>[2x]MGSSHHHHHHLEVLFQGPAGSMATERDQEIIDFIDQGNYTYAQSLITKKLAKSPQKLFYHVLQNEIHLKSGQRELAIKKNLELLNRYPNDPLTIEKLSDFFSKMEMEKESSLVYENAIKKYPVSTETLCLSWFDNSIEKYDFKVFNRIFMYLNKNGKSRLHTLWYAFSFHLLLQEGETDKASLYNSLGKKLMEGLQPFENTQEIYVYTLFLSSKEIEQVLSGVTLPLDLELKLLYMKAMKENASFEALHAYTEKLLFKEKFDDFDTWKLWILSGKEIGKSFEELDQKLTLPTRNISLLKIELDILYSRNIETSVENYYQKFNTKLCCYADLSQYELPTSFIGSLKNSTSEENLITVVNNRKFVNQTDNWDVYERFSTKEGAEYDSNPVNELTLRTIVSDLDSSPQNTIKNIVLLKHLLEQDKYNYKLKLWLMKLYSQLNTNDLIFPIYNGLKIRM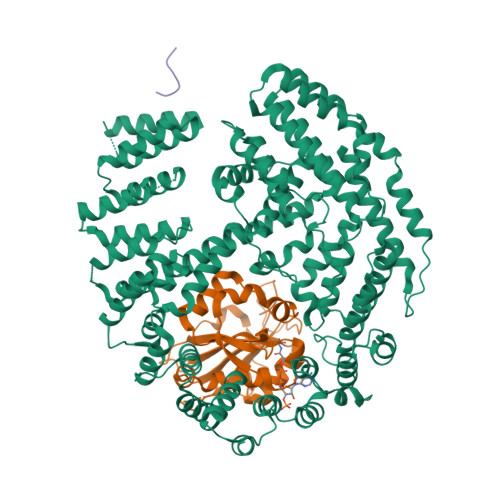TQHETLNYYLTTTNPSKINLDAWVDIYRFYLTSKQEIKESIIQGFDNGVFNKLEGFINFSKRMQNSISLNFTVAKILQISTILGTDGYLNYFIHYLKTNEALIVSDYTDNRDFKSEWNGLEKIDCIDVPVNDVATKLKLLVYSIVFEDQDASRLLKVFNKITSNAKFSVFDNLLYKLYFNLLKITKTKLNPQETQSLYNYLQKNLKTDKLKILIPENLLSGELTQNLTNLVEFIKIVKLLAKRHPSSYMNQLVNLVKPFGKEFKNLKLVQRQHEIIDSMDFEPPISVDISQTKLEIKSSIEDCVVALLNSL;>MTSIKPFQMEDLFELNPVNLDPLTENFNVSFYSQYLIEWPQLFYKSVETPNGQASGYMMAKTEGQLSKKEWHTHITAVTVLDQYRRIGLASKLCLELENLTQVKDTLFIDLFVKVTNTLGRILYEKLGYSVFRRVVGYYGREIQKDRNKIDDSVDAFDMRKLLPRDVNNETVRENGEKVYVLPNEIVF[2x];>[2x]XMDSEVAALVID> VETIELKRG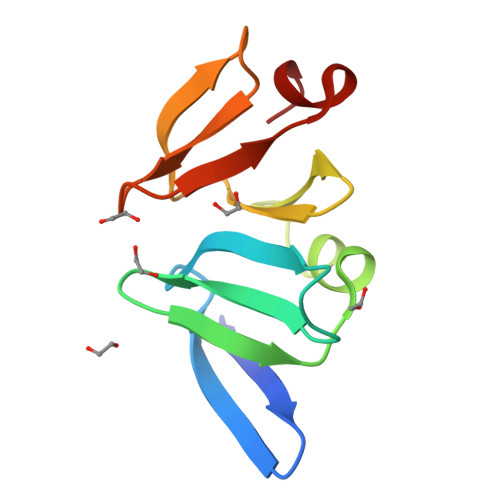SNSVYVQYDDIMFFESSTKSHRLIAHLDNRQIEFYGNLKELSQLDDRFFRCHNSFVVNRHNIESIDSKERIVYFKNKEHCYASVRNVKKI>MQPIPDVNQRIARISAHLHPPKSQMEESSALRRANCRAKGGAPGFKVAILGAAGGIGQPLAMLMKMNPLVSVLHLYDVVNAPGVTADISHMDTGAVVRGFLGQQQLEAALTGMDLIIVPAGVPRKPGMTRDDLFKINAGIVKTLCEGIAKCCPRAIVNLISNPVNSTVPIAAEVFKKAGTYDPKRLLGVTMLDVVRANTFVAEVLGLDPRDVDVPVVGGHAGVTILPLLSQVKPPSSFTQEEISYLTDRIQNGGTEVVEAKAGAGSATLSMAYAAVKFADACLRGLRGDAGVIECAFVSSQVTELPFFASK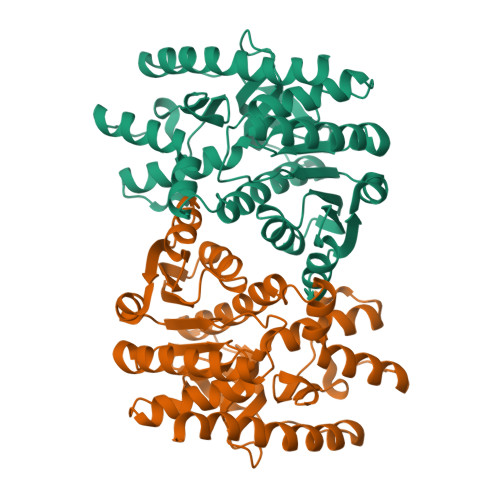VRLGRNGIEEVYSLGPLNEYERIGLEKAKKELAGSIEKGVSFIRSHHHHHH[2x]>[3x]GMEPFKQQKVEDFYDIGEELGSGQFAIVKKCREKSTGLEYAAKFIKKRQSRASRRGVSREEIEREVSILRQVLHHNVITLHDVYENRTDVVLILELVSGGELFDFLAQKESLSEEEATSFIKQILDGVNYLHTKKIAHFDLKPENIMLLDKNIPIPHIKLIDFGLAHEIEDGVEFKNIFGTPEFVAPEIVNYEPLGLEADMWSIGVIT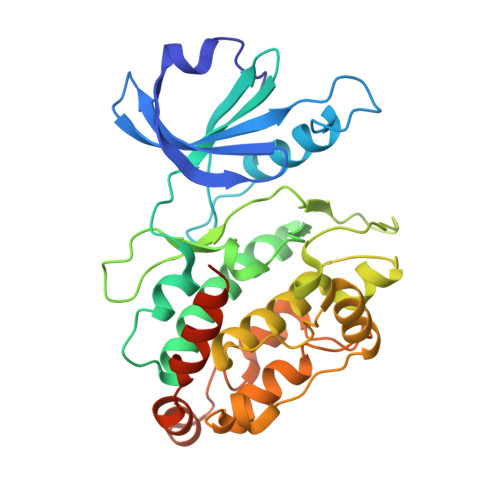YILLSGASPFLGDTKQETLANITSVSYDFDEEFFSHTSELAKDFIRKLLVKETRKRLTIQEALRHPWITPVDNQQAMVRRESVVNLENFRKQYVRRRSKLAFSIVSLCNHLTR> APLVHHHHHHALDENLYFQGALADVSRPPHARKTGGSSPETKYDQPPKCDISGKEAISALSRAKSKHCRQEIGETYCRHKLGLLMPEKVTRFCPLEGKANKNVQWDEDSVEYMPANPVRIAFVLVVHGRASRQLQRMFKAIYHKDHFYYIHVDKRSNYLHRQVLQVSRQYSNVRVTPWRMATIWGGASLLSTYLQSMRDLLEMTDWPWDFFINLSAADYPIRTNDQLVAFLSRYRDMNFLKSHGRDNARFIRKQGLDRLFLECDAHMWRLGDRRIPEGIAVDGGSDWFLLNRRFVEYVTFSTDDLVTKMKQFYSYTLLPAESFFHTVLENSPHCDTMVDNNLRITNWNRKLGCKCQYKHIVDWCGCSPNDFKPQDFHRFQQTARPTFFARKFEAVVNQEIIGQLDYYLYGNYPAGTPGLRSYWENVYDEPDGIHSLSDVTLTLYHSFARLGLRRAETSLHTDGENSCRYYPMGHPASVHLYFLADRFQGFLIKHHATNLAVSKLETLETWVMPKKVFKIASPPSDFGRLQFSEVGTDWDAKERLFRNFGGLLGPMDEPVGMQKWGKGPNVTVTVIWVDPVNVIAATYDILIESTAEFTHYKPPLNLPLRPGVWTVKILHHWVPVAETKFLVAPLTFSNRQPIKPEEALKLHNGPLRNAYMEQSFQSLNPVLSLPINPAQVEQARRNAASTGTALEGWLDSLVGGMWTAMDICATGPTACPVMQTCSQTAWSSFSPDPKSELGAVKPDGRLR;> QEEEGSAGGQGG

The first enzyme in the pathway, peptide O-xylosyltransferase (XT, EC 2.4.2.26), catalyzes the transfer of xylose from uridine diphosphate (UDP)-α-D-xylose onto serine and thus determines the site(s) of GAG attachment on the core protein. XT1 and XT2 are type II transmembrane proteins consisting of a short amino-terminal region facing the cytosol, a single transmembrane helix, a stem region required for Golgi localization (Schön et al., 2006), a catalytic GT-A domain (Lairson et al., 2008, Müller et al., 2006), and a unique C-terminal domain of unknown function, termed “Xylo_C” in the Pfam database (Finn et al., 2008). XT1 has a two-lobed structure, with one lobe comprising the catalytic GT-A domain and the other comprising the Xylo_C domain. To better understand the initial step of GAG biosynthesis, we have determined crystal structures of human XT1 complexed with UDP-xylose and various PG-derived acceptor peptides.

To visualize how the different amino acid substitutions are accommodated in the peptide binding cleft, we selected five variants of the bikunin-derived peptide for structure analysis (peptides 3–7). Three bikunin variants bound identically to the wild-type peptide: peptide 3 (proline at position −3), peptide 5 (alanine at position +1), and peptide 7 (proline at position +3). Position +1 has a strong preference for small amino acids (G, A, S, T, C; note that serine may act as an alternative acceptor). The limited range of amino acids permitted at the position +1 is readily explained by the shape of the peptide binding cavity, which features a narrow constriction on the C-terminal side of the acceptor serine. The structure with peptide 5 shows that the extra methyl group of alanine can be accommodated at this position, but larger side chains would prevent the acceptor serine OH group from reaching the xylose C1 atom. Curiously, all but one of the known GAG attachment sites have a glycine in position +1, even though XT1 works equally well with glycine or alanine. A constriction within the peptide binding cleft requires the acceptor serine to be followed by glycine or alanine.> MESKKRQWALEDFEIGRPLGKGKFGNVYLAREKQSKFILALKVLFKAQLEKAGVEHQLRREVEIQSHLRHPNILRLYGYFHDATRVYLILEYAPLGTVYRELQKLSKFDEQRTATYITELANALSYCHSKRVIHRDIKPENLLLGSAGELKIANFGWSVHAPSSRRTTLCGTLDYLPPEMIEGRMHDEKVDLWSLGVLCYEFL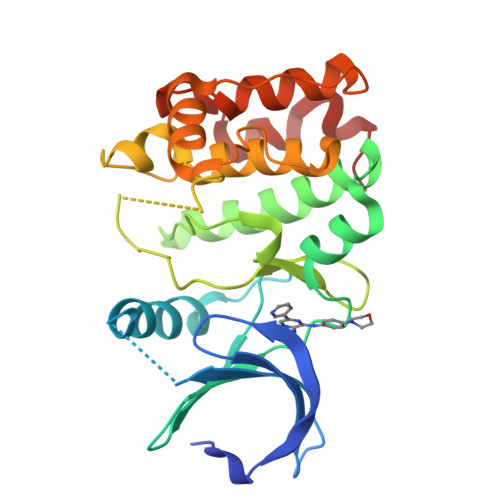VGKPPFEANTYQETYKRISRVEFTFPDFVTEGARDLISRLLKHNPSQRPMLREVLEHPWITANSSKPSN> DQCASSPCQNGGSCKDQLQSYICFCLPAFEGRNCETHKDDQLICVNENG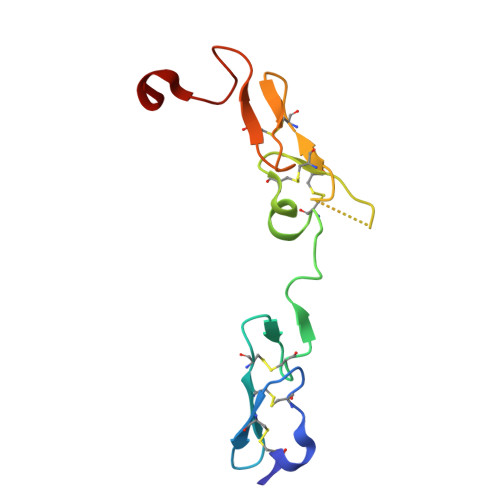GCEQYCSDHTGTKRSCRCHEGYSLLADGVSCTPTVEYPCGKIPILEK>[2x]GSTSMSATR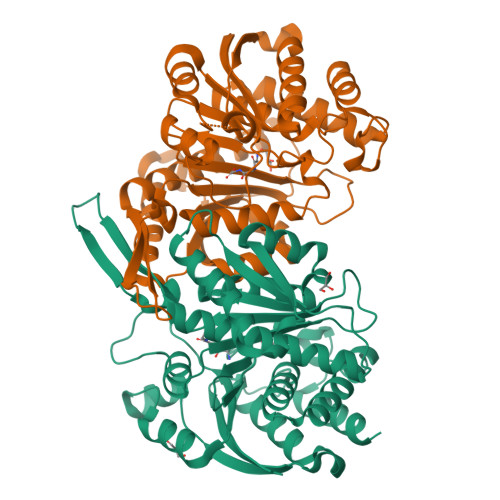RIVLGLIPADGIGKEVVPAARRLMENLPAKHKLKFDFIDLDAGWGTFERTGKALPERTVERLKTECNAALFGAVQSPTHKVAGYSSPIVALRKKMGLYANVRPVKSLDGAKGKPVDLVIVRENTECLYVKEERMVQNTPGKRVAEAIRRISEEASTKIGKMAFEIAKSRQKIRESGTYSIHKKPLVTIIHKSNVMSVTDGLFRESCRHAQSLDPSYASINVDEQIVDSMVYRLFREPECFDVVVAPNLYGDILSDGAASLIGSLGLVPSANVGDNFVMSEPVHGSAPDIAGRGIANPVATFRSVALMLEFMGHQDAAADIYTAVDKVLTEGKVLTPDLGGKSGTNEITDAVLANIHN>[8x]NLPNIVILATGGTIAGSAAANTQTTGYKAGALGVETLIQAVPELKTLANIKGEQVASIGSENMTSDVLLTLSKRVNELLARSDVDGVVITHGTDTLDESPYFLNLTVKSDKPVVFVAAMRPATAISADGPMNLYGAVKVAADKNSRGRGVLVVLNDRIGSARFISKTNASTLDTFKAPEEGYLGVIIGDKIYYQTRLDKVHTTRSVFDVTNVDKLPAVDIIYGYQDDPEYM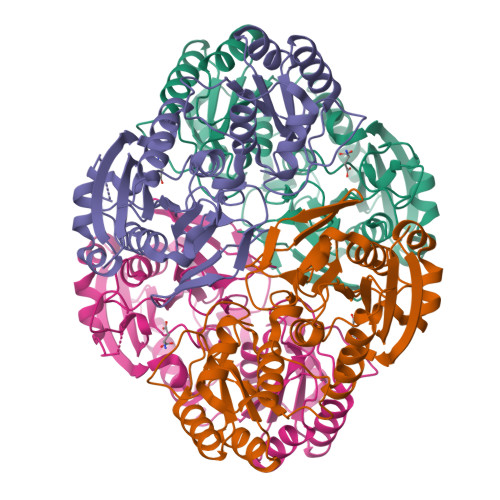YDASIKHGVKGIVYAGMGAGSVSKRGDAGIRKAESKGIVVVRSSRTGSGIVPPDAGQPGLVADSLSPAKSRILLMLALTKTTNPAVIQDYFHAY>[2x]SNAKDVLGLTLLEKTLKERLNLKDAIIVSGDSDQSPWVKKEMGRAAVACMKKRFSGKNIVAVTGGTTIEAVAEMMTPDSKNRELLFVPARGGLGEDVKNQANTICAHMAEKASGTYRLLFVPGQLSQGAYSSIIEEPSVKEVLNTIKSASMLVHGIGEAKTMAQRR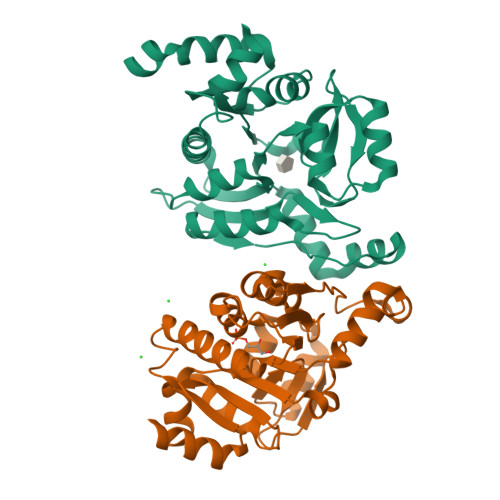NTPLEDLKKIDDNDAVTEAFGYYFNADGEVVHKVHSVGMQLDDIDAIPDIIAVAGGSSKAEAIEAYFKKPRNTVLVTDEGAAKKLLRDE>[2x]DTIYKMNKSTRGIAVIINNKDFLRSSGMDRYPRNGTDVDRDALAKLFRALKFDVRIYNNQTRAEIRRITKEMAITNHTPYDAFIFSILTHGEEGVIYGTDGTMAIKDLTAIFKDCTTLVGKPKMFFFQACQGHEYMDGVSVPAEADFVYAYSTVPGYYSWRNSVNGSWFIQSLTKVFEENAERMDILRMLTRVNAMVSTYKSRTGDYYSDSKRQVSSVVSMLRKELYFFPENV;> KLFSFGG;>XDEVD[2x]

To gain insight into caspase activity and regulation in coral, we expressed and characterized two caspases each from two species of Caribbean reef-building corals, Orbicella faveolata and Porites astreoides. Two proteins referred to as PaCasp7a and OfCasp3a based on sequences similarity to human caspases contain CARD motifs at the N terminus, an unusual combination that has not been observed in caspases-3 or -7 enzymes from higher eukaryotes, and indeed these proteins function as initiator caspases. Our functional characterization suggests that PaCasp7a and OfCasp3a may function similarly to caspase-2 because they exhibit DXXDase activity and contain an N-terminal CARD motif. We also report the first X-ray crystal structure of a coral caspase, that of PaCasp7a determined at 1.57 Å resolution, which reveals an N-terminal peptide bound near the active site that may serve as a regulatory exosite.

We attempted to crystalize all four of the coral caspases, and we were successful in obtaining diffraction quality crystals of PaCasp7a with an inhibitor (DEVD-CHO) bound in the active site. The crystals diffracted in the P212121 space group, and we determined the structure to high resolution at 1.57 Å. The data show that the PaCasp7a is very similar to human caspases, with a root mean square deviation of <1 Å compared with HsCasp3. In the active site, the carboxylate group of the P4 aspartate hydrogen bonds to Asn315 (CP-162) on active site loop 3 (L3), the backbone amide of Arg356 (GP9-02) on L4, and through water–hydrogen bonds to Trp321 (CP-168) (on L3) as well as the backbone carbonyl of Arg356 (GP9-02) (on L4). In general, the active site provides hydrophilic binding pockets for the P3 glutamate and P4 aspartate of the substrate, and a more hydrophobic binding pocket for the P2 valine side chain, similarly to that of HsCasp3. The structure of PaCasp7a with inhibitor bound shows that the insertion extends the loop compared with HsCasp3 and results in an “RYP” motif in L1 near the catalytic histidine. The structure of PaCasp7a also reveals a peptide bound on the protein surface near α-helices 1 and 4. The structure shows that amino acids in the N terminus of PaCasp7a (N′-AKLFSFGG-C′) (N′-PD-A025 to PD-G018-C′ in the common position numbering) compose the peptide, where the two phenylalanine side chains bind in a hydrophobic pocket between helices 1 and 4. The binding pocket on the protein is formed by five hydrophobic residues on the two helices (Leu187 (CP-031), Ala190 (CP-034), Leu191 (CP-035), Phe330 (CP-177), Ala334 (CP-181)) as well as Phe381 and Phe382 (CP-217 and CP-218) at the C terminus.>DYDQLQNKPDLGAFAQKEETNSKITKLESSKADKSAVYSKAESKIELDKKLSLTGGIVTGQLQFKPNKSGIKPSSSVGGAINIDMSKSEGAAMVMYTNKDTTDGPLMILRSDKDTFDQSAQFVDYSGKTNAVNIVMRQPSAPNFSSALNITSANEGGSAMQIRGVEKALGTLKITHENPNVEAKYDENAAALSIDIVKKQKGGKGTAAQGIYINSTSGTA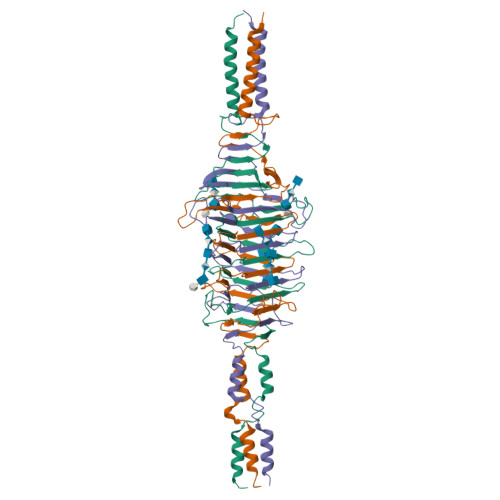GKMLRIRNKNEDKFYVGPDGGFHSGANSTVAGNLTVKDPTSGKHAATKDYVDEKIAELKKLILKKLEHHHHHH[3x]> VKPISPEQEELIHRLVYFQNEYEQPSDEDLKRISNTPSEGEDQSDLNFRHITEITILTVQLIVEFAKRLPGFDKLLREDQIALLKACSSEVMMLRMARRYDVGSDSILFANNQPYTRDSYSLAGMGETVDDLLRFCRQMYGMKVDN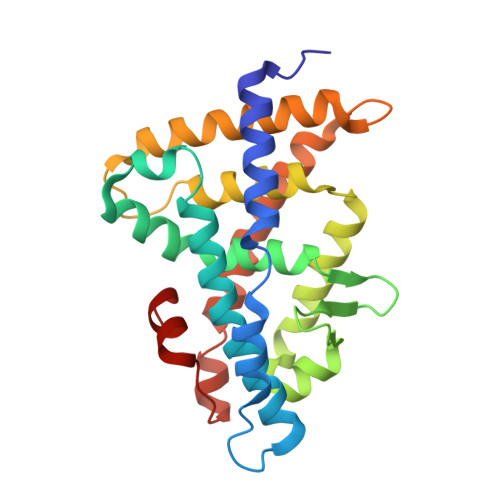AEYALLTAIVIFSERPSLIEGWKVEKIQEIYLEALKVYVDNRRKPASGTIFAKLLSVLTELRTLGNLNSEMCFSLKLKNKKLPPFLAEIWDV2-[[2-methoxy-4-(2-oxidanylidenepyrrolidin-1-yl)phenyl]amino]-4-(oxan-4-ylamino)-7H-pyrrolo[2,3-d]pyrimidine-5-carbonitrile 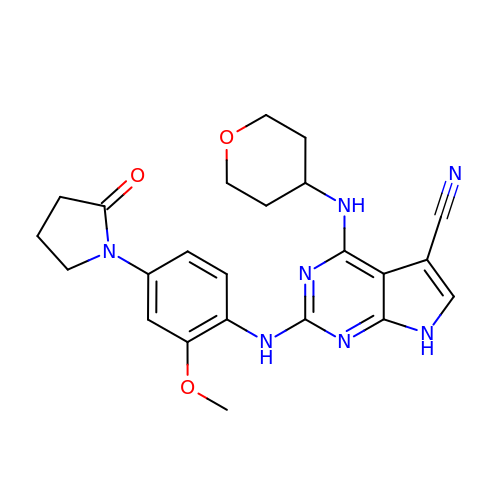| C23 H25 N7 O3 | GWQWEYUZUSIHAO-UHFFFAOYSA-N>[2x]SNAFRRKLTALDYHNPAGFNCKDETEFRNFIVWLEDQKIRHYKIEDRGNLRNIHSSDWPKFFEKYLRDVNCPFKIQDRQEAIDWLLGLAVRLEYGDNAEKYKD

The human RtcB ligase ortholog RTCB, also referred to as HSPC117 or FAAP, is part of an essential heteropentameric tRNA ligase complex (tRNA-LC), along with the DEAD-box helicase DDX1, as well as FAM98B, CGI-99 (also known as RTRAF or hCLE), and ASHWIN (ASW). The tRNA ligase complex is an essential factor for both tRNA biogenesis and XBP1 mRNA splicing during the unfolded protein response in human cells. By contrast, the RtcB ligases are GTP-dependent enzymes that catalyze the direct joining of RNA strands with terminal 2′,3′>P and 5′-OH. RTCB is the only subunit of tRNA-LC that is essential and sufficient for RNA ligation, but it requires the protein cofactor Archease for multiple-turnover catalysis.

Structural modeling using Phyre2 and PCOILS servers predicted that both CGI-99 and FAM98B comprised N-terminal calponin homology (CH)-like domains followed by putative C-terminal coiled-coil regions (Schou et al., 2014). To verify this experimentally, we determined the crystal structure of the N-terminal domain of CGI-99 comprising residues Phe2-Asp101CGI-99 at a resolution of 2.0 Å. The protein construct adopts a globular fold connected via a flexible linker to an N-terminal α-helix comprising residues Phe2–Asn18CGI-99, which is stabilized in different conformations in the two molecules present in the asymmetric unit by crystal packing interactions. Our structural analysis reveals that the CH-like domain of CGI-99 exhibits closest structural homology to the microtubule binding NDC80-like family of CH domains, as proposed by an earlier study. The N-terminal domain of CGI-99 (Phe2-Asp101CGI-99) was able to co-precipitate a minimal FAM98B construct spanning residues Arg2-Lys184FAM98B, indicating that the CGI-99:FAM98B interaction is dependent on both the N-terminal CH domain and a predicted beta-hairpin motif (residues Glu145-Lys184FAM98B) in FAM98B, and the N-terminal CH domain in CGI-99. Taken together, these results indicate that the formation of the CGI-99:FAM98B heterodimer is mediated by the respective N-terminal regions of the subunits and suggest that the N-terminal CH-like domains of CGI-99 and FAM98B may comprise an independently functioning module within tRNA-LC. In addition, the CGI-99 and FAM98B subunits of tRNA-LC form a stable heterodimer through an independent interaction interface involving their N-terminal domains. This heterodimer further serves as an interaction platform for the recruitment of ASW, the fifth tRNA-LC subunit. There is, however, no evidence to date to indicate that CGI-99 and FAM98B, or indeed tRNA-LC, interact with MTs or other cytoskeletal proteins.>[2x]SLRLHAGVWGLKVRYEGSFEVSK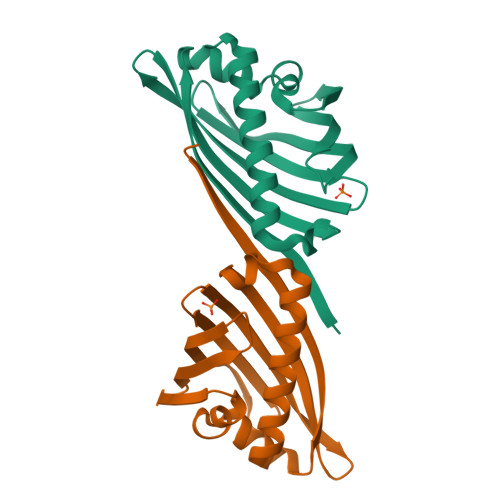TPEEVFEFLTDPKRFSRAFPGFKSVEVEDGSFTIELRLSLGPLRGDARVRASFEDLEKPSKATVKGSGRGAGSTLDFTLRFAVEPSGGGSRVSWVFEGNVGGLAASMGGRVLDSLARRMINDVISGVKRELGEA>[4x]TDVVIVSAARTAVGKFGGSLAKIPAPELGAVVIKAALERAGVKPEQVSEVIMGQVLTAGSGQNPARQAAIKAGL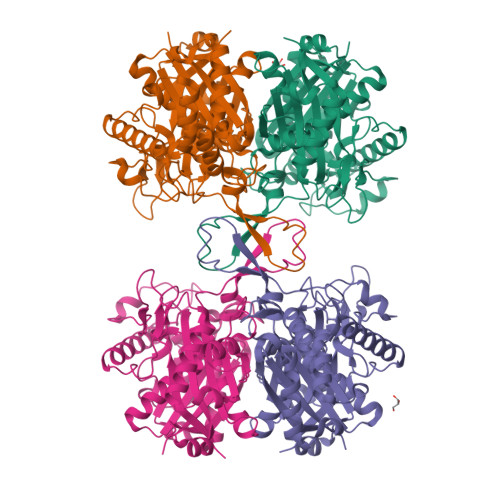PAMVPAMTINKVCGSGLKAVMLAANAIMAGDAEIVVAGGQENMSAAPHVLPGSRDGFRMGDAKLVDTMIVDGLWDVYNQYHMGITAENVAKEYGITREAQDEFAVGSQNKAEAAQKAGKFDEEIVPVLIPQRKGDPVAFKTDEFVRQGATLDSMSGLKPAFDKAGTVTAANASGLNDGAAAVVVMSAAKAKELGLTPLATIKSYANAGVDPKVMGMGPVPASKRALSRAEWTPQDLDLMEINEAFAAQALAVHQQMGWDTSKVNVNGGAIAIGHPIGASGCRILVTLLHEMKRRDAKKGLASLCIGGGMGVALAVERK> MNAKKRKGSAVERNIVSRLRDKGFAVVRAPASGSKRKD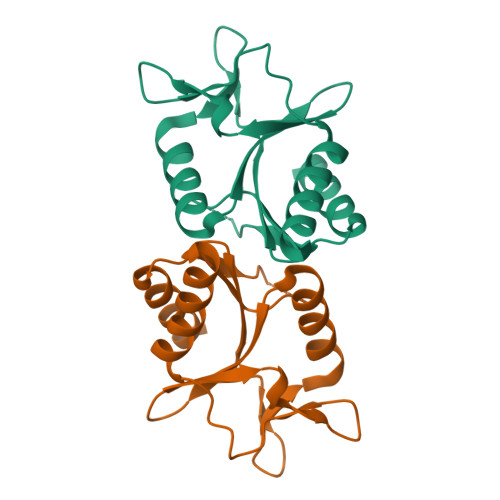PIPDIIALKNGVIILIEMKSRKDIEGKIYVRREQAEGIIEFARKSGGSLFLGVKKPGVLKFIPFEKLRRTETGNYVADSEIEGLDLEDLVRLVEAKISRTLDNFL>[2x]MVLPDIKKGKDMINILPFEIISRNTKTLLITYISSVDITHEGMKKVLESLRSKQGIISE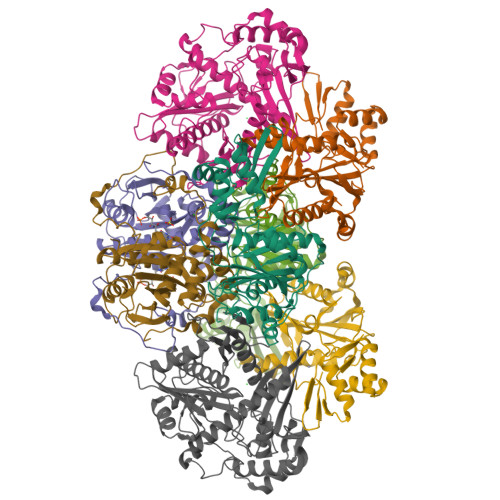YLLDKLLDESLIDKDKGKEFLITTGVINKTKTSPLWVNSVIISDVPHLFSNAREQWKCDGVFVSHIIDIKDNNINVSDSTLIWLHLENYHSDIVKRIYSKFESNPGVAFIQSYYLKESFRIDGVYSPDLGTPCHFCHIERWLSREEKSFRRNEMSWANLLQLLKKYQMTLPALALGESERGFSYHLIKRRLQELTGTSLVKSHVDNFMSSVSADLITCILCKEPVIHWQACSCLER;> MSKHELSLVEVTHYTDPEVLAIVKDFHVRGNFASLPEFAERTFVSAVPLAHLEKFENKEVLFRPGFSSVINISSSHNFSRERLPSGINFCDKNKLSIRTIEKLLVNAFSSPDPGSVRRPYPSGGALYPIEVFLCRLSENTENWQAGTNVYHYLPLSQALEPVATCNTQSLYRSLSGGDSERLGKPHFALVYCIIFEKALFKYRYRGYRMALMETGSMYQNAVLVADQIGLKNRVWAGYTDSYVAKTMNLDQRTVAPLIVQFFGDVNDDKCLQ;> MINVYSNLMSAWPATMAMSPKLNRNMPTFSQIWDYERITPASAAGETLKSIQGAIGEYFERRHFFNEIVTGGQKTLYEMMPPSAAKAFTEAFFQISSLTRDEIITHKFKTVRAFNLFSLEQQEIPAVIIALDNITAADDLKFYPDRDTCGCSFHGSLNDAIEGSLCEFMERQSLLLYWLQGKANTEISSEIVTGINHIDEILLALRSEGDIRIFDITLPGAPGHAVLTLYGTKNKISRIKYSTGLSYANSLKKALCKSVVELWQSYICLHNFLIGGYTDDDIIDSYQRHFMSCNKYESFTDLCENTVLLSDDVKLTLEENITSDTNLLNYLQQISDNIFVYYARERVSNSLVWYTKIVSPDFFLHMNNSGAININNKIYHTGDGIKVRESKMVPFP> MAATNMTDNVTLNNDKISGQAWQAMRDIGMSRFELFNGRTQKAEQLAAQAEKLLNDDSTDWNLYVKSDKKAPVEGDHYIRINSSITVAEDYLPAGQKNDAINKANQKMKEGDKKGTIEALKLAGVSVIENQELIPLQQTRKDVTTALSLMNEGKYYQAGLLLKSAQDGIVVDSQSVQLEHHHHHH

We characterized various features of the Salmonella-derived YfdX protein, including the crystal structure that contains a novel fold, previously unknown stoichiometric features, proof of contribution to antibiotic response, and participation in the control of bacterial virulence. Moreover, we found that Salmonella YfdX plays a significant role in bacterial susceptibility to penicillin G and carbenicillin and is involved in the negative regulation of bacterial virulence in an insect larvae model. Collectively, these data indicate that the recombinant st_YfdX protein can form a dimer or tetramer in solution, and this process is affected by pH of the solution. No homologous protein was identified in this search except for kp_YfdX (Z-score 20.1): a number of proteins containing a helical bundle were listed including Nitrosomonas europaea small metal-binding protein (Z-score 9.9) and E. coli cytochrome b562 (Z-score 8.5), but their structures overlapped with the st_YfdX structure only partially, indicating that YfdX adopts a novel protein fold that has not been identified yet.

Rectangular crystals (space group F222) diffracted to the resolution of 1.4 Å were obtained in a crystallization condition with pH 4.6 (Crystal I), implying that this crystal might consist of the st_YfdX tetramer. Its asymmetric unit contains a single st_YfdX molecule that is composed of six α-helices, one 310-helix, and three β-strands. One 310-helix is located in the middle of the α2–β1 loop. Of note, we figured out that a tetramer-shaped oligomeric form of st_YfdX is shown in our crystal lattice, which can be fairly well-matched to that of kp_YfdX. In contrast, we could not find any crystallographic evidence for the formation of a st_YfdX trimer in our structure. We next structurally analyzed the intermolecular binding between st_YfdX monomers in the tetrameric form. The two st_YfdX molecules designated as Mol A and Mol B in Figure 3 interact with each other mainly through very tight hydrophobic contacts. Hydrophobic interactions provide additional force for the complex formation between Mol A and Mol C, which are mediated by Tyr100 and Ile137 from one molecule and Pro81′′, Tyr87′′, Leu158′′, Leu170′′, Val179′′, and the hydrocarbon part of Thr154′′, Lys163′′, and Gln166′′ from the opposite molecule (right). Overall, the interaction between Mol A and Mol B mainly depends on tight hydrophobic interaction and appears to be tight and dense, whereas that between Mol A and Mol C is maintained by the combination of hydrogen bonds and loose hydrophobic interaction but seems to be relatively weak and detachable.Centrioles have proximal-distal polarity and a 9-fold radial symmetry imparted by a likewise symmetrical central scaffold, the cartwheel. The spindle assembly abnormal protein 6 (SAS-6) self-assembles into 9-fold radially symmetric ring-shaped oligomers that stack via an unknown mechanism to form the cartwheel. SAS-6 proteins comprise a globular “head” domain at their N-terminus followed by a long coiled coil that mediates stable protein homo-dimerization (Keller et al., 2014), and a disordered C-terminal extension. The characteristic shape of the SAS-6 ring led to the proposal that the protein head domains comprise the central “hub” of the centriolar cartwheel, with SAS-6 coiled coils forming the cartwheel “spokes” (Cottee et al., 2015; Kitagawa et al., 2011; van Breugel et al., 2011; van Breugel et al., 2014; Yoshiba et al., 2019).

In contrast, structures of the CrSAS-6_CCMiddle fragment, resolved from two different crystal forms, revealed parallel complexes featuring extensive interaction interfaces between coiled-coil domains, within each crystal’s asymmetric unit. CrSAS-6_CCMiddle form II, resolved to 2.43 Å using one copy of the CrSAS-6_CCMiddle coiled coil from form I as molecular replacement model, featured four copies of the coiled-coil domain per asymmetric unit. Of these, two copies were arranged in a symmetric-interacting fashion identical to the form I complex. In striking contrast, the remaining two CrSAS-6 coiled-coil copies formed a parallel but distinctly asymmetric complex driven by hydrogen-bonding and ionic interactions, which buried ∼1,700 Å2 of solvent-accessible surface. The symmetry break was caused by an ∼8-Å shift between the two coiled-coil copies, resulting from a 5-Å translation along the coiled-coil length and a 35° relative rotation. The contact interface of the asymmetric CrSAS-6 coiled-coil complex overlapped to a great extent with that of the symmetric complex, but also involved additional amino acid residues; a comparison of amino acids at the two interfaces is shown in Figure S2B. Hydrophobic contacts were limited to packing of the H294 side chain against G297′ and G301ʹ (prime denotes amino acids of the second coiled-coil copy in the complex), which form part of a GxxxG motif known for mediating interactions between α-helices (Kleiger et al., 2002), and sidechain interactions between A340-A336ʹ and V351 with the aliphatic part of S347ʹ. Specifically, we substituted residues V351E/D361N (CrSAS-6_CCVD), thereby abrogating a mild hydrophobic (V351-S347′) and an ionic (R367-D361′) contact of the asymmetric interface. Although CrSAS-6VD did form cartwheels, they were less abundant and less apparent compared with those formed by the WT protein, suggesting reduced stacking propensity.

>GPKLREVKYELDTKVSELSHKLGSSEGSNRSLEEETARLRSLNQQLSSSKHELEIQLNEAKAKVLALDEKAQSQGDVIEQQRGRLRDMEAALRQTEQRCADLRDTLASAEGRAKEA[8x]> MGSSHHHHHHSQDPMAPPVRYCIPGERLCNLEEGSPGSGTYTRHGYIFSSLAGCLMKSSENGALPVVSVVRETESQLLPDVGAIVTCKVSSINSRFAKVHILYVGSMPLKNSFRGTIRKEDVRATEKDKVEIYKSFRPGDIVLAKVISLGDAQSNYLLTTAENELGVVVAHSESGIQMVPISWCEMQCPKTHTKEFRKVAR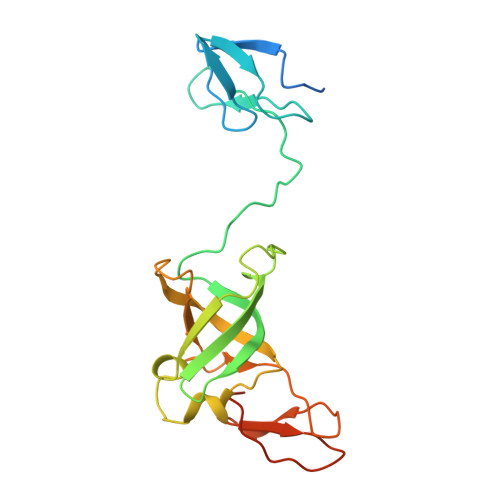VQPEFLQT>[6x]MDTIAARALTVMRACATLQEARIVLEANVMEILGIAINRYNGLTLRGVTMRPTSLAQRNEMFFMCLDMMLSAAGINVGPISPDYTQHMATIGVLATPEIPFTTEAANEIARVTGETSTWGPARQPYGFFLETEETFQPGRWFMRAA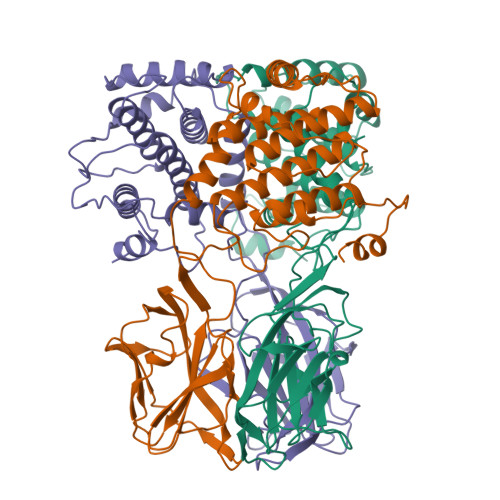QAVTAVVCGPDMIQVSLNAGARGDVQQIFQGRNDPMMIYLVWRRIENFAMAQGNSQQTQAGVTVSVGGVDMRAGRIIAWDGQAALHVHNPTQQNAMVQIQVVFYISMDKTLNQYPALTAEIFNVYSFRDHTWHGLRTAILNRTTLPNMLPPIFPPNDRDSILTLLLLSTLADVYTVLRPEFAIHGVNPMPGPLTRAIARAAYV>MGSDKIHHHHHHMNDFKNQWLRKRTFAIPASRLTGRLTTLKSDVPAADSLFWKLWNGSLDTAVQVLQTDYFKGIAAGTLDPNAYGSLMVQDGYYCFRGRDDYATAATCAQDET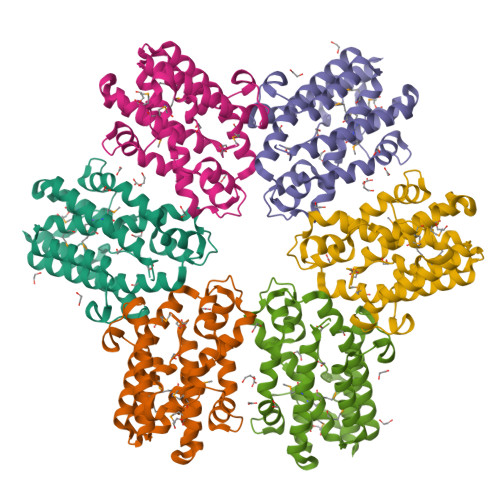LREFFKAKAKSYDEYNETYHQTWHLREASGLIPGTDIKDYADYEAYVAGSLASPYMCVVMLPCEYLWPWIANFLDGYTPTNSLYRFWIEWNGGTPNGAYQMGNMLEQYRDKIDEDKAVEIFNTAMNYELKVFTSSTILTTIENGK[2x]2-ETHYL-4(1H)-QUINOLINONE 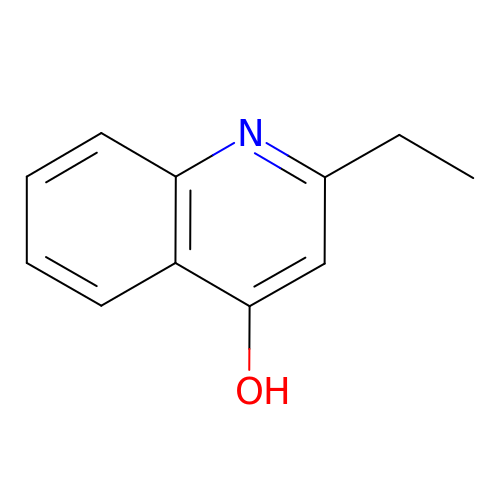| C11 H11 N O | YBKUKKHOCTXYGB-UHFFFAOYSA-N> GGCGAAGAAC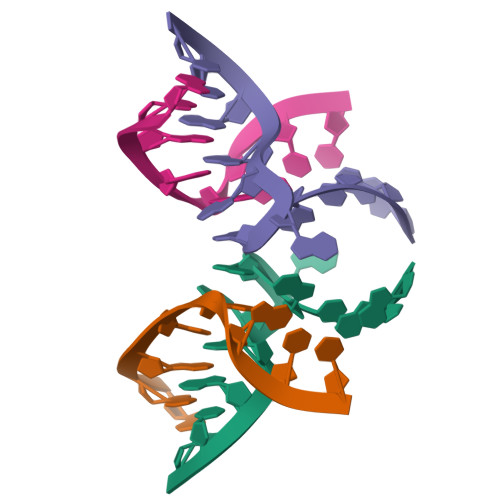U;> GGGGAGCU propan-2-amine | C3 H9 N | 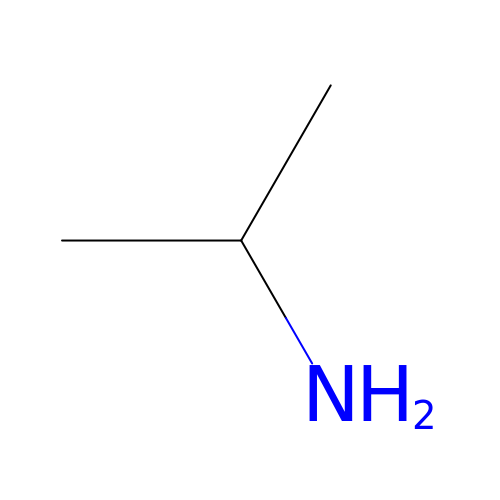JJWLVOIRVHMVIS-UHFFFAOYSA-N>[2x]MHHHHHHLEVLFQGPQTSEYYQEAANPIATNPALWAKVTAPQISWGSTDIRYKKEEPAPIHSAQKSMNLTAWKGEKISAQLVVWTPKVLNDLTFMVSDLTSGSATISKENIRTGFVRYVITDELNKDGLGACGYRNSADFDSTLVADVIDHITPTLTLPANSTQGGWISVNIPQGTKAGKYTGTVTVKADGITLSELKLNLQVKNRTLPPPSEWAFHLDLWQNPYAVSRYYNVEPFSKKHFDLMRPLMKLYADAGGKVITASIMHKPWNGQTYDAFESMVTWLKKADGTWYFDYTVFDKWVEFMMDLGVKKQISCYSMVPWRLSFQYFDQASNSFKFLDAKPGEVAYEEFWMNMLQDF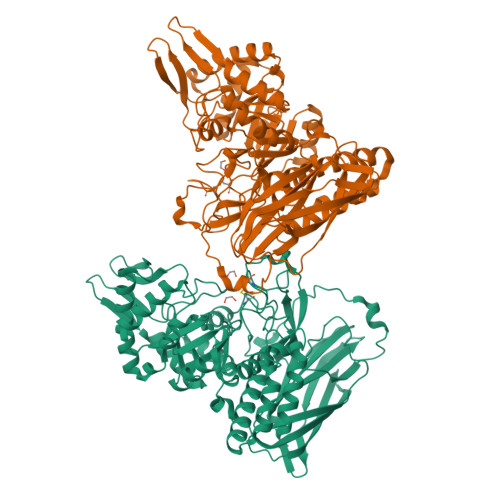SKHLKAKGWFDITHIAMDERPMKDMQETLKVIRKADKDFKVSLAGTYHKELLDDLNDYCITIAEKFTPEEIEARRKAGKVTTYYTCCTEPRPNTFTFSEPAEAEWLAWHSAKENLDGYLRWALNSWVKNPLQDSRFTAWAAGDTYMIYPGARSSIRLERLTEGIQFFEKVRILKEEFEEKGNKGAIKNIDKTLKMFDESSMDKISPTTAVNKAKKVINRY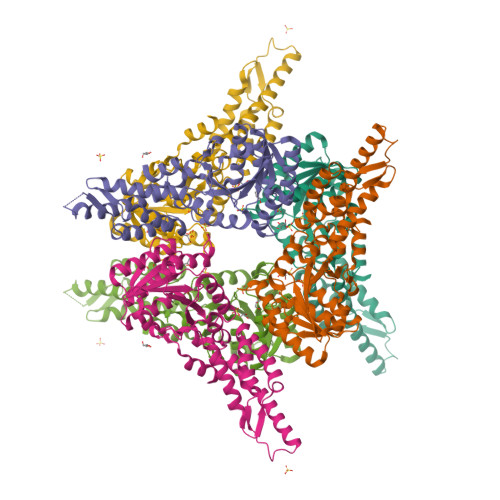>[3x]GSHMASMFGKLREKLKSFVKRVEEEVEKEEEEVEKKGLLDRILTVEIKEKDVDKALDELEIDLLEADVALEVVDALREKIKQKLVGKKVRIGTDKGKIIEEAVKEAVSEILETSRRIDLIEEIRKAEKPYVIMFVGFNGSGKTTTIAKLANWLKNHGFSVVIAASDTFRAGAIEQLEEHAKRIGVKVIKHSYGADPAAVAYDAIQHAKARGIDVVLIDTAGRSETNRNLMDEMKKIARVTKPNLVIFVGDALAGNAIVEQARQFNEAVKIDGIILTKLDADARGGAALSISYVIDAPILFVGVGQGYDDLRPFEKEWFLERIFGEENA> MSIADQSLAKRVQGVSQQAIDEGRIVGSVVLIARHGRVIYANASGYADREQKKPMVRETQFRLSSVSKPYITLAAMRMIEQQKLGLDDTVSRWLPWFTPALADGVRPPIKIRHLLSHTAGLDYRLSQPAEGPYHRLGIKDGMELSSLTLEQNLRLLAQADLLAEPGSEFRYSLAIDVLGAVLEQVAGEPLPQVFNHWVAQPLGLRNTGFYTTDVDNLATAYHDTAAEPEPIRDGMLLTLPEGFGFEIELAPSRALDAQAYPSGGAGMVGDADDVLQLVETLRTGKEGILQPATAALMRQAHVGSHAETQGPGWGFGFGGAVLEDAQLAATPQHNGTLQWGGVYGHSWFYDPQAA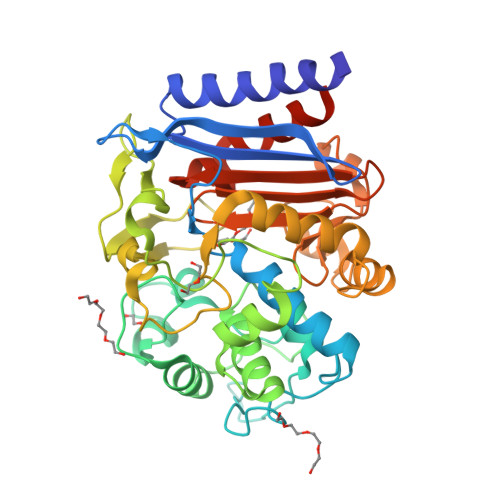ISVVALTNTAFEGMSGRYPLQIRDAVYGTNEPTRGGHHHHHH> ESAWGPAATIAARQSATGTKTDTPIQKVPQSISVVTAEEMALHQPKSVKEALSYTPGVSVGTRGASNTYDHLIIRGFAAEGQSQNNYLNGLKLQGNFYNDAVIDPYMLERAEIMRGPVSVLYGKSSPGGLLNMVSKRPTTEPLKEVQFKAGTDSLF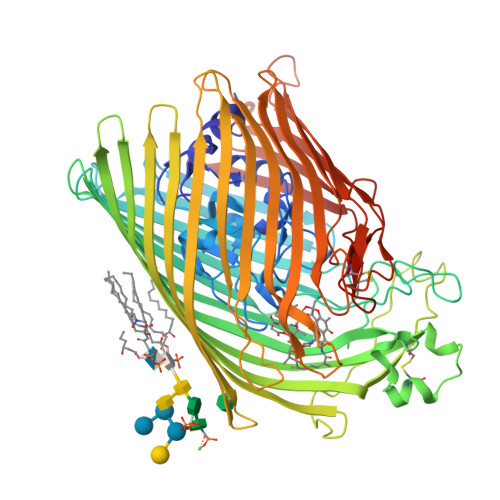QTGFDFSDSLDDDGVYSYRLTGLARSANAQQKGSEEQRYAIAPAFTWRPDDKTNFTFLSYFQNEPETGYYGWLPKEGTVEPLPNGKRLPTDFNEGAKNNTYSRNEKMVGYSFDHEFNDTFTVRQNLRFAENKTSQNSVYGYGVCSDPANAYSKQCAALAPADKGHYLARKYVVDDEKLQNFSVDTQLQSKFATGDIDHTLLTGVDFMRMRNDINAWFGYDDSVPLLNLYNPSSHHHHHHGSSVNTDFDFNAKDPANSGPYRILNKQKQTGVYVQDQAQWDKVLVTLGGRYDWADQESLNRVAGTTDKRDDKQFTWRGGVNYLFDNGVTPYFSYSESFEPSSQVGKDGNIFAPSKGKQYEVGVKYVPEDRPIVVTGAVYNLTKTNNLMADPEGSFFSVEGGEIRARGVEIEAKAALSASVNVVGSYTYTDAEYTTDTTYKGNTPAQVPKHMASLWADYTFFDGPLSGLTLGTGGRYTGSSYGDPANSFKVGSYTVVDALVRYDLARVGMAGSNVALHVNNLFDREYVASCFNTYGCFWGAERQVVATATFRF>[3x]GPPLPEELVLLERTLADGSTEQIIFSSAGDVNVYDLQALCDKVGWPRRPLTKIAASLRNSYLVATLHSVTMPSKAEGEERKQLIGMARATSDHAFNATIWDVLVD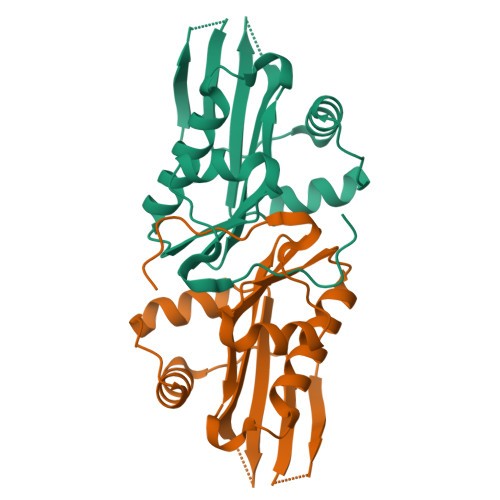PSYQGQGLGKALMEKVIRTLLQRDISNITLFADNKVVDFYKNLGFEADPQGIKGMFWYPRF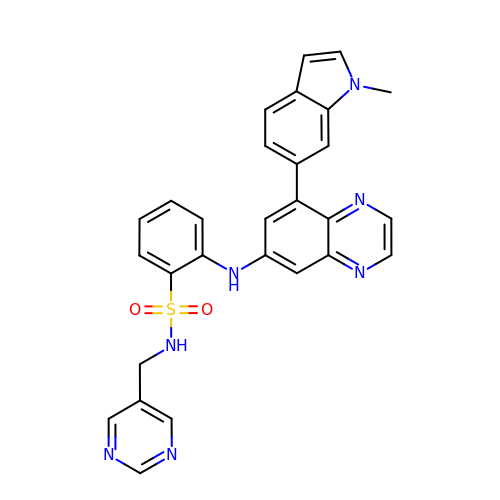2-[[8-(1-methylindol-6-yl)quinoxalin-6-yl]amino]-~{N}-(pyrimidin-5-ylmethyl)benzenesulfonamide | C28 H23 N7 O2 S | FHKKLQIBTXYWGR-UHFFFAOYSA-N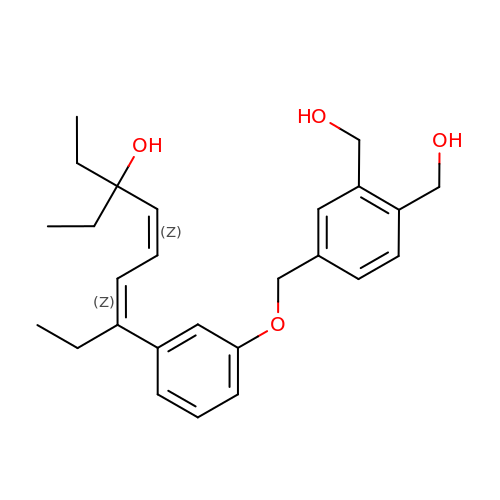(4E,6Z)-7-(3-{[3,4-bis(hydroxymethyl)benzyl]oxy}phenyl)-3-ethylnona-4,6-dien-3-ol | C26 H34 O4 | ZPQGIRYXMGFFNL-PKSQTMKJSA-N>MPPNNSKYVLDPVSIKSVCGGEESYIRCVEYGKKKAHYSNLNLLAKAILAGMFVGLCAHASGIAGGLFYYHKLREIVGASMSVFVYGFTFPIAFMCIICTGSDLFTGNTLAVTMALYEKKVKLLDYLRVMTISLFGNYVGAVSFAFFVSYLSGAFTNVHAVEKNHFFQFLNDIAEKKVHHTFVECVSLAVGCNIFVCLAVYFVLTLKDGAGYVFSVFFAVYAFAIAGYEHIIANIYTLNIALMVNTKITVYQAYIKNLLPTLLGNYIAGAIVLGLPLYFIYKEHYYNFER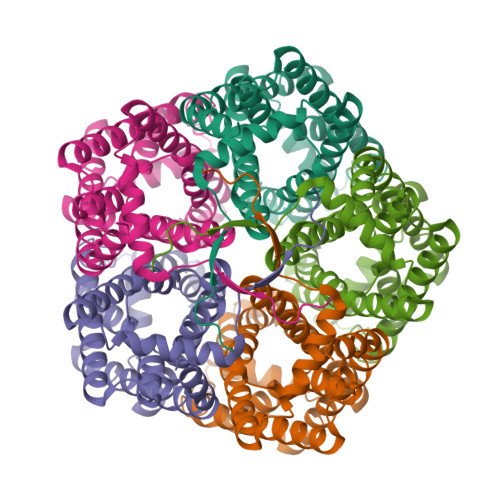SKRDNNDAQMKSLSIELRN[5x]>MGNVDLVFLFDGSMSLQPDEFQKILDFMKDVMKKLSNTSYQFAAVQFSTSYKTEFDFSDYVKWKDPDALLKHVKHMLLLTNTFGAINYVATEVFREELGARPDATKVLIIITDGEATDSGNIDAAKDIIRYIIGIGKHFQTKESQETLHKFASKPASEFVK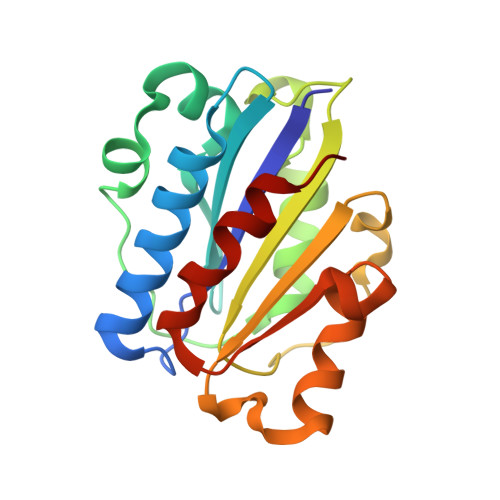ILDTFEKLKDLFTELQKKIY[3x]> XGELKAIAQELKAIAKELKAI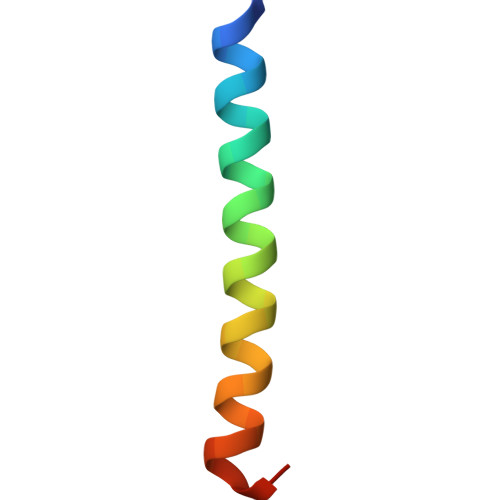AWEHKAIAQGAGX> LDIPA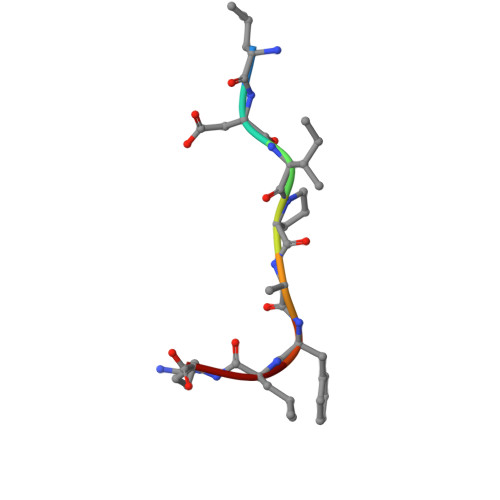FLR1-(3-{5-[4-(aminomethyl)phenyl]-1H-pyrrolo[2,3-b]pyridin-3-yl}phenyl)-3-(2-phenoxyphenyl)urea 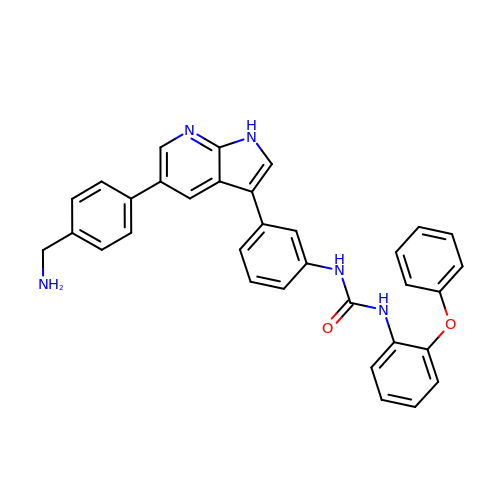| C33 H27 N5 O2 | KSTUYVHCHCYOAB-UHFFFAOYSA-N>[2x]GAMASSNTAATNADSAWLEAQEEEEVGFPVRPQVPLRPMTYKAALDISHFLKEKGGLEGLIWSQRRQEILDLWIYHTQGYFPDWQNYTPGPGIRYPLTFGWCFKLVPVEPEKVEEANEGENNSLLHPMSLHGMEDAEKEVLVWRFDSKLAFHHMARELHPEYYKDA;>[2x]MEDIIVVALYDYVSWSPDDLSFQKGDQMVVLEESGEWWKARSLATRKEGYIPSNYVARVDSGGGTSGGGRH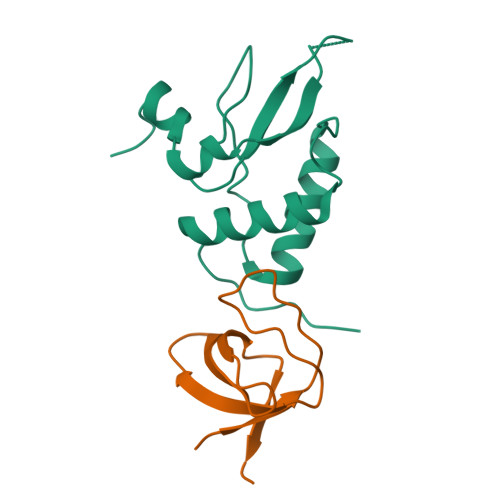RRRQAERMSQIKRLLSEKK>MDSSEVVKVKQASIPAPGSILSQPNTEQSPAIVLPFQFEATTFGTAETAAQVSLQTADPITKLTAPYRHAQIVECKAILT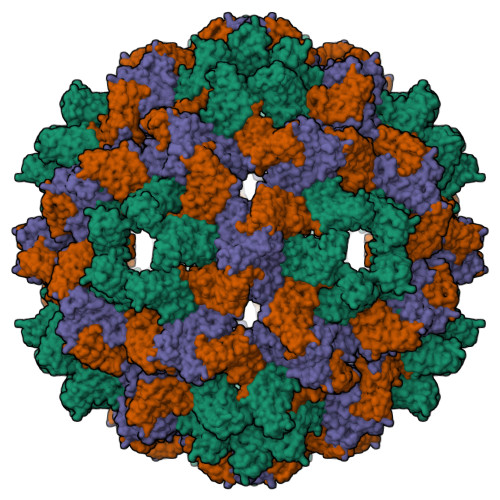PTDLAVSNPLTVYLAWVPANSPATPTQILRVYGGQSFVLGGAISAAKTIEVPLNLDSVNRMLKDSVTYTDTPKLLAYSRAPTNPSKIPTASIQISGRIRLSKPMLIAN[3x]2-[[3-[(3-azanyl-2,2-dimethyl-propyl)carbamoyl]phenyl]amino]-~{N}-(2-chloranyl-6-methyl-phenyl)-1,3-thiazole-5-carboxamide 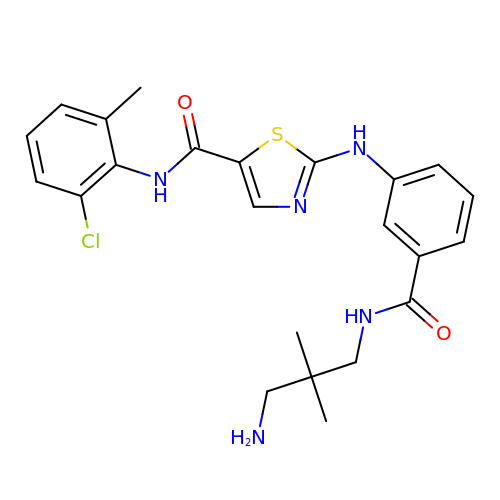| C23 H26 Cl N5 O2 S | DVESFPFOHKUMHP-UHFFFAOYSA-N>[2x]DLLVPKLTASVTDGAVGVTVDAPVSVTAADGVLAAVTMVNDNGRPVAGRLSPDGLRWSTTEQLGYNRRYTLNATALGLGGAATRQLTFQTSSPAHLTMPYVMPGDGEVVGVGEPVAIRFDENIADRGAAEKAIKITTNPPVEGAFYWLNNREVRWRPEHFWKPGTAVDVAVNTYGVDLGEGMFGEDNVQTHFTI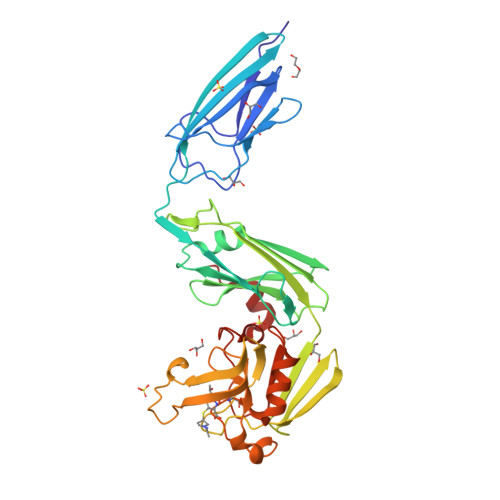GDEVIATADDNTKILTVRVNGEVVKSMPTSMGKDSTPTANGIYIVGSRYKHIIMDSSTYGVPVNSPNGYRTDVDWATQISYSGVFVHSAPWSVGAQGHTNTSHGCLNVSPSNAQWFYDHVKRGDIVEVVNTVGGTLPGIDGLGDWNIPWDQWRAGNAK> ETFPPKYLHYDEETSHQLLCDKCPPGTYLKQHCTAKW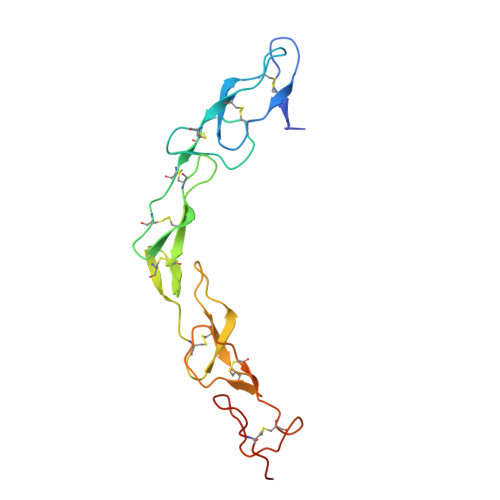KTVCAPCPDHYYTDSWHTSDECLYCSPVCKELQYVKQECNRTHNRVCECKEGRYLEIEFCLKHRSCPPGFGVVQAGTPERNTVCKRCPDGFFSNETSSKAPCRKHTNCSVFGLLLTQKGNATHDNICSHHHHHH>GCGUUUGAAACGC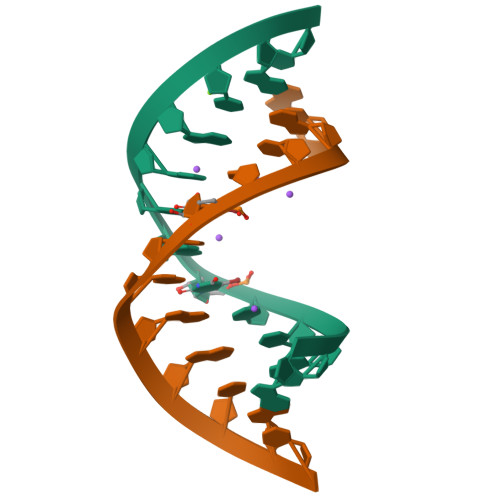[2x]> MMSMIEKLKKFTQIPGISGYEERIREEIIREIKDFADYKVDAIGNLIVELGEGEERILFMAHMDEIGLLITGITDEGKLRFRKVGGIDDRLLYGRHVNVVTEKGILDGVIGATPPHLSLERDK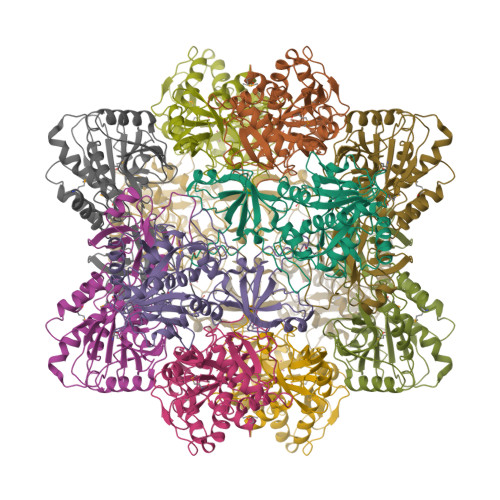SVIPWYDLVIDIGAESKEEALELVKPLDFAVFKKHFSVLNGKYVSTRGLDDRFGVVALIEAIKDLVDHELEGKVIFAFTVQEEVGLKGAKFLANHYYPQYAFAIDSFACCSPLTGDVKLGKGPVIRAVDNSAIYSRDLARKVWSIAEKNGIEIQIGVTGGGTDASAFQDRSKTLALSVPIKYLHSEVETLHLNDLEKLVKLIEALAFEL> XMEEKLKKSKIIFVVGGPGSGKGTQCEKIVQKYGYTHLSTGDLLRAEVSSGSARGKMLSEIMEKGQLVPLETVLDMLRDAMVAKVDTSKGFLIDGYPREVKQGEEFERKIGQPTLLLYVDAGPETMTKRLLKRGETSGRVDDNEETIKKRLETYYKA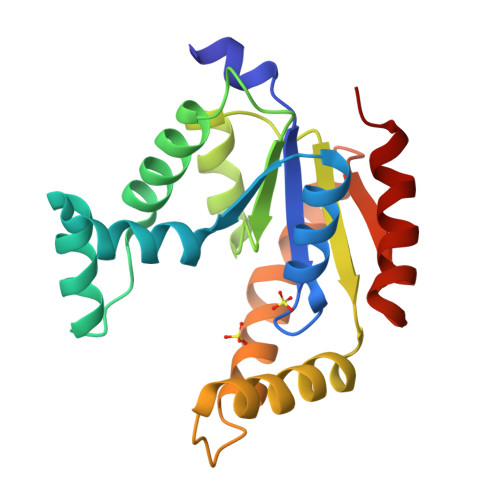TEPVIAFYEKRGIVRKVNAEGSVDDVFSQVCTHLDTLK>GQSITDYNYKKPLHNDYQILDKSKIFGSNSGSFVMYSMKKDKYYIYNEKESRKRYSPNSTYKIYLAMFGLDRHIINDENSRMSWNHKHYPFDAWNKEQDLNTAMQNSVNWYFERISDQIPKNYTATQLKQLNYGNKNLGSYKSYWMEDSLKISNLEQVIVFKNMMEQNNHFSKKAKNQLSSSLLIKKNEKYELYGKTGTGIVNGKYNNGWFVGYVITNHDKYYFATHLSDGKPSGKNA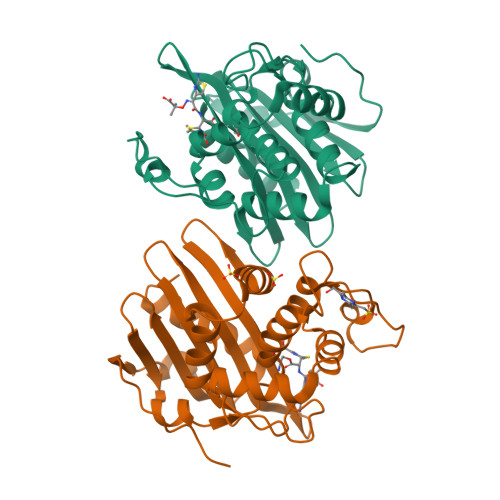ELISEKILKEMGVLNGQ[4x]>[2x]MSHTILLVQPTKRPEGRTYADYESVNECMEGVCKMYEEHLKRMNPNSPSITYDIS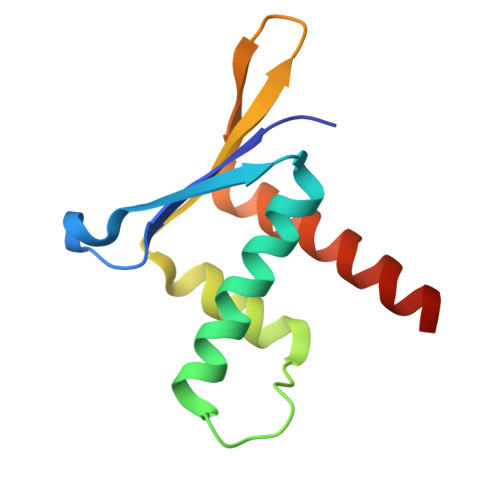QLFDFIDDLADLSCLVYRADTQTYQPYNKDWIKEKIYVLLRRQAQQAGK> MASGSCQGCEEDEETLKKLIVRLNNVQEGKQIETLVQILEDLLVFTYSEHASKLFQGKNIHVPLLIVLDSYMRVASVQQVGWSLLCKLIEVCPGTMQSLMGPQDVGNDWEVLGVHQLILKMLTVHNASVNLSVIGLKTLDLLLTSGKITLLILDEESDIFMLIFDAMHSFPANDEVQKLGCKALHVLFERVSEEQLTEFVENKDYMILLSALTNFKDEEEIVLHVLHCLHSLAIPCNNVEVLMSGNVRCYNIVVEAMKAFPMSERIQEVSCCLLHRLTLGNFFNILVLNEVHEFVVKAVQQYPENAALQISALSCLALLTETIFLNQDLEEKNENQENDDEGEEDKLFWLEACYKALTWHRKNKHVQEAACWALNNLLMYQNSLHEKIGDEDGHFPAHREVMLSMLMHSSSKEVFQASANALSTLLEQNVNFRKILLSKGIHLNVLELMQKHIHSPEVAESGCKMLNHLFEGSNTSLDIMAAVVPKILTVMKRHETSLPVQLEALRAILHFIVPGMPEESREDTEFHHKLNMVKKQCFKNDIHKLVLAALNRFIGNPGIQKCGLKVISSIVHFPDALEMLSLEGAMDSVLHTLQMYPDDQEIQCLGLSLIGYLITKKNVFIGTGHLLAKILVSSLYRFKDVAEIQTKGFQTILAILKLSASFSKLLVHHSFDLVIFHQMSSNIMEQKDQQFLNLCCKCFAKVAMDDYLKNVMLERACDQNNSIMVECLLLLGADANQAKEGSSLICQVCEKESSPKLVELLLNSGSREQDVRKALTISIGKGDSQIISLLLRRLALDVANNSICLGGFCIGKVEPSWLGPLFPDKTSNLRKQTNIASTLARMVIRYQMKSAVEEGTASGSDGNFSEDVLSKFDEWTFIPDSSMDSVFAQSDDLDSEGSEGSFLVKKKSNSISVGEFYRDAVLQRCSPNLQRHSNSLGPIFDHEDLLKRKRKILSSDDSLRSSKLQSHMRHSDSISSLASEREYITSLDLSANELRDIDALSQKCCISVHLEHLEKLELHQNALTSFPQQLCETLKSLTHLDLHSNKFTSFPSYLLKMSCIANLDVSRNDIGPSVVLDPTVKCPTLKQFNLSYNQLSFVPENLTDVVEKLEQLILEGNKISGICSPLRLKELKILNLSKNHISSLSENFLEACPKVESFSARMNFLAAMPFLPPSMTILKLSQNKFSCIPEAILNLPHLRSLDMSSNDIQYLPGPAHWKSLNLRELLFSHNQISILDLSEKAYLWSRVEKLHLSHNKLKEIPPEIGCLENLTSLDVSYNLELRSFPNEMGKLSKIWDLPLDELHLNFDFKHIGCKAKDIIRFLQQRLKKAVPYNRMKLMIVGNTGSGKTTLLQQLMKTKKSDLGMQSATVGIDVKDWPIQIRDKRKRDLVLNVWDFAGREEFYSTHPHFMTQRALYLAVYDLSKGQAEVDAMKPWLFNIKARASSSPVILVGTHLDVSDEKQRKACMSKITKELLNKRGFPAIRDYHFVNATEESDALAKLRKTIINESLNFKIRDQLVVGQLIPDCYVELEKIILSERKNVPIEFPVIDRKRLLQLVRENQLQLDENELPHAVHFLNESGVLLHFQDPALQLSDLYFVEPKWLCKIMAQILTVKVEGCPKHPKGIISRRDVEKFLSKKRKFPKNYMTQYFKLLEKFQIALPIGEEYLLVPSSLSDHRPVIELPHCENSEIIIRLYEMPYFPMGFWSRLINRLLEISPYMLSGRERALRPNRMYWRQGIYLNWSPEAYCLVGSEVLDNHPESFLKITVPSCRKGCILLGQVVDHIDSLMEEWFPGLLEIDICGEGETLLK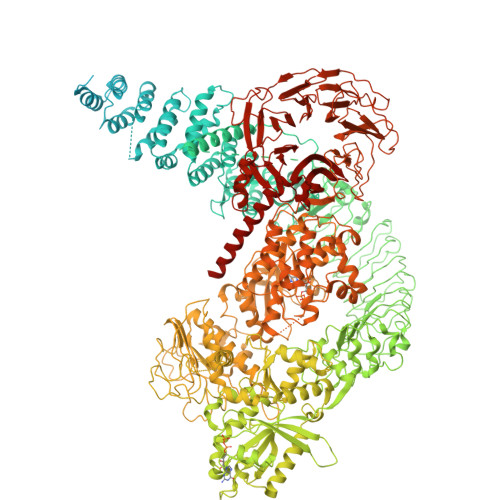KWALYSFNDGEEHQKILLDDLMKKAEEGDLLVNPDQPRLTIPISQIAPDLILADLPRNIMLNNDELEFEQAPEFLLGDGSFGSVYRAAYEGEEVAVKIFNKHTSLRLLRQELVVLCHLHHPSLISLLAAGIRPRMLVMELASKGSLDRLLQQDKASLTRTLQHRIALHVADGLRYLHSAMIIYRDLKPHNVLLFTLYPNAAIIAKIADYGIAQYCCRMGIKTSEGTPGFRAPEVARGNVIYNQQADVYSFGLLLYDILTTGGRIVEGLKFPNEFDELEIQGKLPDPVKEYGCAPWPMVEKLIKQCLKENPQERPTSAQVFDILNSAELVCLTRRILLPKNVIVECMVATHHNSRNASIWLGCGHTDRGQLSFLDLNTEGYTSEEVADSRILCLALVHLPVEKESWIVSGTQSGTLLVINTEDGKKRHTLEKMTDSVTCLYCNSFSKQSKQKNFLLVGTADGKLAIFEDKTVKLKGAAPLKILNIGNVSTPLMCLSESTNSTERNVMWGGCGTKIFSFSNDFTIQKLIETRTSQLFSYAAFSDSNIITVVVDTALYIAKQNSPVVEVWDKKTEKLCGLIDCVHFLREVTVKENKESKHKMSYSGRVKTLCLQKNTALWIGTGGGHILLLDLSTRRLIRVIYNFCNSVRVMMTAQLGSLKNVMLVLGYNRKNTEGTQKQKEIQSCLTVWDINLPHEVQNLEKHIEVRKELAEKMRRTSVE Most eukaryotic proteins are N-terminally acetylated by a set of Nα acetyltransferases (NATs). Here, we report Naa50 homologs from the filamentous fungi Chaetomium thermophilum and Neurospora crassa with significant N- and C-terminal extensions to the conserved GNAT domain. Structural and biochemical analyses show that CtNaa50 shares the GNAT structure and substrate specificity with other homologs. However, in contrast to previously analyzed Naa50 proteins, it does not form NatE.

In order to characterize the CtNaa50 GNAT domain, we crystallized CtNaa5082-289 in complex with the bisubstrate analog (peptide sequence: M1pV2pN3pA4pL5p) and solved its X-ray crystal structure. Crystals of CtNaa5082-289/CoA-Ac-MVNAL belong to space group P212121 with one molecule per asymmetric unit and diffracted to 1.1 Å resolution. CtNaa5082-289 shares the GCN5-related N-acetyltransferase (GNAT) fold with a mixture of four α helices and seven β strands. The conserved AcCoA-binding motif Q/RxxGxG/A in turn β4 to α3 comprises residues RSLGLA in CtNaa50 and interacts with the pyrophosphate part of CoA. The major differences are in three loop regions β2–β3, β3–β4, and α3–β5, which are longer than in orthologous Naa50 proteins. In particular, loop β3–β4 has a length of 32 residues, which is 30 residues longer than the human protein. This loop could be completely built and due to crystal packing folds back to the protein with the Q175 side-chain pointing towards the substrate peptide entry site. The peptide moiety of CoA-Ac-MVNAL binds at the substrate peptide binding site, while the two Naa50 loops, α1–α2 and β6–β7, connected by van der Waals contacts, fold over the peptide. Several residues surround M1p to create a hydrophobic binding pocket, which is typical for active Naa50 enzymes: L107, P108, and V109 in loop α1–α2, and Y264 and L267 in loop β6–β7 as well as W237 in β5. The active site of CtNaa5082-289 includes a tightly bound water molecule, which is important for acetylation and is also present in other active Naa50 structures.

> MGLPSGASIVPLAQEHIPALRRINSLLLPVAYPDSFYHKALDPLASGLFSRAILWQDTNADPPKVVGGLICRLEPNPFLSVTGEPTPVQLPADQPQRAPQAPKDTPFHAIYIQSLALLSPYRSLGLAAAALDHIIATAAVLPAAGSNIDARTIYAHVWTENEEGLKWYESRGFVKEGGEPVKGYYFKLRPDTAWIVRRHIGESAKLNDVVHHHHHH;> MVNAL>[2x]GPAEALEWTWVEFTVDETVDVVVCMMYSPGEFYCHFLKDDALEKLDDLNQSLADYCAQKPPNGFKAEIGRPCCAFFSGDGNWY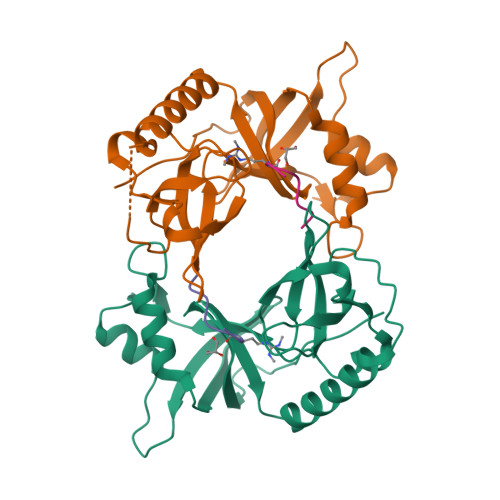RALVKEILPSGNVKVHFVDYGNVEEVTTDQLQAILPQFLLLPFQGMQCWLVDIQPPNKHWTKEATARFQACVVGLKLQARVVEITANGVGVELTDLSTPYPKIISDVLIREQLVLRCG;>GRAGPAGRGLVFR[2x]>GAMGKVTHSIHIEKSDTAADTYGFSLSSVEEDGIRRLYVNSVKETGLASKKGLKAGDEILEINNRAADALNSSMLKDFLSQPSLG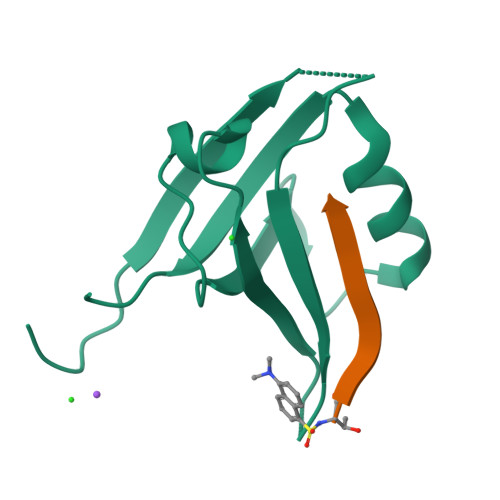LLVRTYPEL[2x];>[2x]TKQEEFYA>GKSRQRSPAN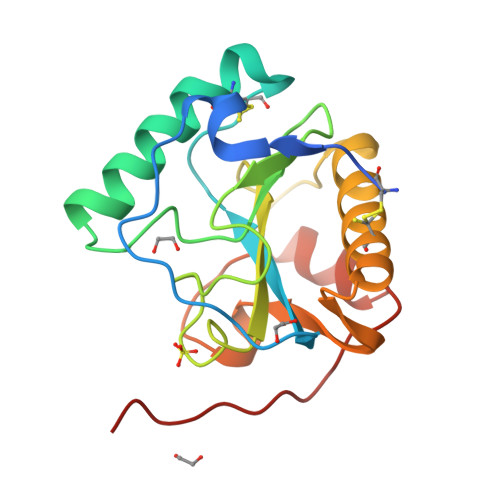CPTIKLKRQWGGKPSLGLHYQVRPIRYVVIHHTVTGECSGLLKCAEILQNMQAYHQNELDFNDISYNFLIGNDGIVYEGTGWGLRGAHTYGYNAIGTGIAFIGNFVDKLPSDAALQAAKDLLACGVQQGELSEDYALIAGSQVISTQSPGLTLYNEIQEWPHWLSNPHHHHHH[2x]> GHMSFVITNPEALTVAATEVRRIRDRAIQSDAQ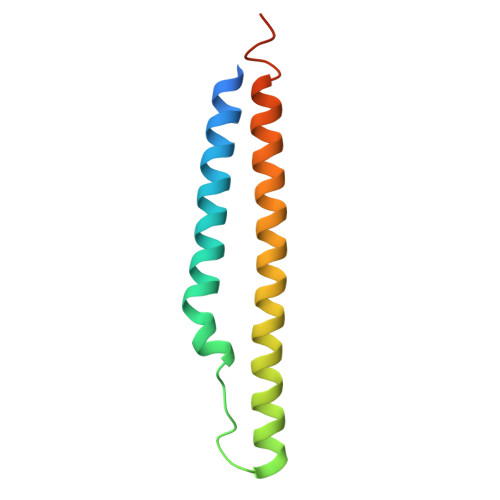VAPMTTAVRPPAADLVSEKAATFLVEYARKYRQTIAAAAVVLEEFAHALTTGADKYATAEADNIKTFS> MTTVSCPANVITTTESDRIAGLFNIPAGIIPTGNVLSTIEVCAHRCIFDFFKQIRSDDNSLYSAQFDILLGTYCNTLNFVRFLELGLSVACICTKFPELAYVRDGVIQFEVQQPMIARDGPHPVDQPVHNYMVKRIHKRSLSAAFAIASEALSLLSNTYVDGTEIDSSLRIRAIQQMARNLRTVLDSFERGTADQLLGVLLEKAPPLSLLSPINKFQPEGHLNRVARAALLSDLKRRVCADMFFMTRHAREPRLISAYLSDMVSCTQPSVMVSRITHTNTRGRQVDGVLVTTATLKRQLLQGILQIDDTAADVPVTYGEMVLQGTNLVTALVMGKAVRGMDDVARHLLDITDPNTLNIPSIPPQSNSDSTTAGLPVNARVPADLVIVGDKLVFLEALERRVYQATRVAYPLIGNIDITFIMPMGVFQANSMDRYTRHAGDFSTVSEQDPRQFPPQGIFFYNKDGILTQLTLRDAMGTICHSSLLDVEATLVALRQQHLDRQCYFGVYVAEGTEDTLDVQMGRFMETWADMMPHHPHWVNEHLTILQFIAPSNPRLRFELNPAFDFFVAPGDVDLPGPQRPPEAMPTVNATLRIINGNIPVPLCPISFRDCRGTQLGLGRHTMTPATIKAVKDTFEDRAYPTIFYMLEAVIHGNERNFCALLRLLTQCIRGYWEQSHRVAFVNNFHMLMYITTYLGNGELPEVCINIYRDLLQHVRALRQTITDFTIQGEGHNGETSEALNNILTDDTFIAPILWDCDALIYRDEAARDRLPAIRVSGRNGYQALHFVDMAGHNFQRRDNVLIHGRPVRGDTGQGIPITPHHDREWGILSKIYYYIVIPAFSRGSCCTMGVRYDRLYPALQAVIVPEIPADEEAPTTPEDPRHPLHAHQLVPNSLNVYFHNAHLTVDGDALLTLQELMGDMAERTTAILVSSAPDAGAATATTRNMRIYDGALYHGLIMMAYQAYDETIATGTFFYPVPVNPLFACPEHLASLRGMTNARRVLAKMVPPIPPFLGANHHAT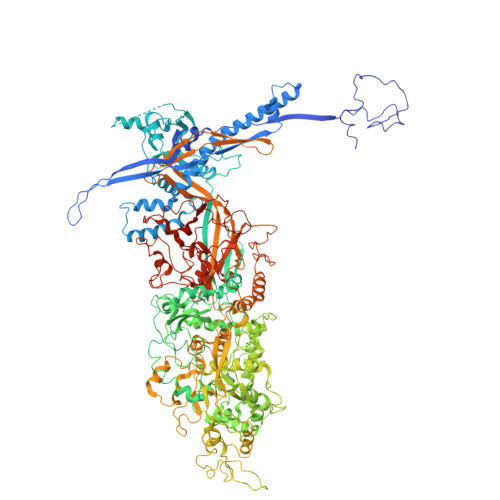IRQPVAYHVTHSKSDFNTLTYSLLGGYFKFTPISLTHQLRTGFHPGIAFTVVRQDRFATEQLLYAERASESYFVGQIQVHHHDAIGGVNFTLTQPRAHVDLGVGYTAVCATAALRCPLTDMGNTAQNLFFSRGGVPMLHDNVTESLRRITASGGRLNPTEPLPIFGGLRPATSAGIARGQASVCEFVAMPVSTDLQYFRTACNPRGRASGMLYMGDRDADIEAIMFDHTQSDVAYTDRATLNPWASQKHSYGDRLYNGTYNLTGASPIYSPCFKFFTPAEVNTNCNTLDRLLMEAKAVASQSSTDTEYQFKRPPGSTEMTQDPCGLFQEAYPPLCSSDAAMLRTAHAGETGADEVHLAQYLIRDASPLRGCLPLPR> MASMGVPALFRLLSRKFAKVITPVIEAPTEKLPDGTEIEPDLSLPNPNGVECDNLYLDMNGIVHPCSHPEDRPAPETEDEMMVAVFEYTDRILAMVRPRQLLFIAIDGVAPRAKMNQQRSRRFRSSREAALKEEELQAFIEEAKQQGI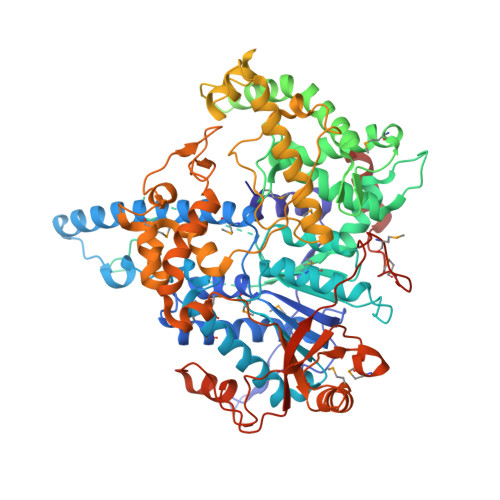PIDENATKKKSWDSNCITPGTPFMDTLAKSLRYYIINKLNSDPCWRNVRFILSDASVPGEGEHKIMEFIRSQRVKPEYDPNTHHVVYGLDADLIMLGLATHEPHFRVLREDVFFQQGSTKKTKEERLGIKRLDDVSETNKVPVKKPFIWLNVSILREYLEVELYVPNLPFPFDLERAIDDWVFFIFFVGNDFLPHLPSLDIRDGAVERLTEIWRASLPHMGGYLTLDGSVNLARAEVILSAVGNQEDDIFKRLKQQEDRRNENYRRRQQRESNQESESYVDNVVIQRSVETQSTEVVTSSKSTSVDTKPPKKTQKIDAPAPVDLVNLSEKTSNRSLGATNRELINNRAANRLGLSREAAAVSSVNKLAASALKAQLVSNETLQNVPLEDSIASSSAYEDTDSIESSTPVVHPIDTKVSNVGQKRKAPDSTEENENTDTVRLYEPGYRERYYEQKFHISPDEPEKIREAVKHYVHGLCWVLLYYYQGCPSWTWYYPYHYAPFAADFKDLASIDVKFELNQPFKPYEQLLGVLPAASKNNLPEKLQTLMTDENSEIIDFYPENFTIDLNGKKFEWQGVALLPFIDENRLLNAVSKIYPQLTEEESKRNEDGSTLLFISEHHPMFSELVKQLYSKKRQGKPLKLSGKMAHGLFGKVNTNDSVIPNVSVQCPIDVTSADALQKYGSIDDNQSISLVFEVPKSHFVHKSMLLRGVKMPNRVLTPEDINQVRAERSFSSRRNNGNSAAALEHHHHHH>MGLNFFRKAAPEVRTEPVAERKASVTGRIVAMASGAGRPVWGPRDTVSLMRTGFAGNPVGFRSVKLIAEATAAVPLICQDAERRYEIHPVLDLLRRPNAGQGRAELFEALIGQILLSGNGYLEAVCPEPGVPRELHVLRSDRMAVVPGADGWPVGYDYTVGGRKHRFDMTGHPDPICHIKSFHPTDDHYGLSPMQAAAVALDVHNAASAWSKALLDNAARPSGAIIYKGADGQGVLAPEQYERLIFEMETHHQGARNAGRPMLLEGGLDWKPMGFSPSDMEFHETKAAAAREIALAFGVPPMLIGIPGDATYANYAEANRAFYRLTVLPLLTRVSAALAWWLSGYLGAQIELKPDLDQVPALAVERDQLWARIGAAGFLSNSEKRVLLGLPPTAEG[2x];>[2x]MMLNEVTAVPGTALPVAEFRDHLRLGTGFADLGAEDAALLSYLRAAIAAIEGRTAKALISRGFRLALTAWRWGDMQTLPIAPVATVTALRLVDAAGVETPVAAGWRLVPDMARPRIEALGAMLPMIPTGGRVEIDFTAGFGASWSALPVDLAQAVFLLAAQYYELRHDGAAEGGAMPFGVMALIERWRTVRVLGGRP;> MSRPRLNRLLVLEEAVRVADGAGGHRLDWQAKGEVWAEVTAGSGSERAGEFVTLASVPFTIVVRAAPVGAARRPRPEQRFREGARIFRILAVAERDREGHYLSCFAREEVVA;> MSYAVAGALQAAVYQQLRADAVLAALVGTAVYDAVPPGPLAGTYVSLGPEDVADASDKTGAGAVHDFVISVITDAAGFATAKAAAAAVSDALVGADLVLSRGRLVGLWFLRAKARRVEKADMRRIDLVFRARVEG;> MAAQNGKDLLIKLDLTGSGQFETIAGLRATRISFNAETVDVTSLESQGGWRELLGGAGVRSASISGAGVFKDADTDERARQIFFDGEVPEFQVIIPDFGIVQGPFMITSIDYAGSHNGEASYELAMASAGALSFTAI

Gene transfer agents (GTAs) are DNA-containing phage-like particles produced by some species of bacteria and archaea. The genes encoding proteins that form Rhodobacter capsulatus GTA particles (RcGTA) are derived from phage DNA, which has been integrated into the bacterial genome. Here, we use cryo-electron microscopy (cryo-EM) to determine the structures of RcGTA before and after DNA ejection, and to visualize the interactions of RcGTA with R. capsulatus cells. Particles of RcGTA have heads with a diameter of 38-nm and 49-nm long tails.

The dodecamer of the adaptor proteins provides the binding site for a hexamer of stopper proteins, resulting in a symmetry mismatch between the two complexes. Adaptor loops from two neighboring adaptor proteins differ in their conformations and interact with one subunit of stopper protein. The first adaptor loop is oriented parallel to the tail axis and fits into a cleft within β-sheets of a stopper protein, whereas the adaptor loop of the second subunit is wedged between two stopper proteins. A hexamer of RcGTA stopper proteins (Rcc01689, g7) binds to the adaptor complex. Each 112-residue-long stopper protein interacts with adaptor loops from two neighboring adaptor proteins. At the distal interface, the long and insertion loops and C-terminus of the stopper protein bind to a terminator protein. However, the long loop of the RcGTA stopper protein interacts with the tail terminator protein and does not block the central tail channel. A hexamer of tail terminator proteins (Rcc01690, g8) binds to the distal interface of the stopper proteins. Unlike other tail proteins of RcGTA, the tail terminator protein contains α-helices 1 and 2 in its N-terminus. α-helix 1 binds to the insertion loop of the stopper protein and α-helix 2 interacts with α-helix 3 from the same tail terminator protein. The insertion and short loops of the tail terminator protein interact with the long and insertion loops of the stopper protein.>[2x]MITDLADNIERLKANDGLKFSQEYESIDPGQQFTWENSNLEVNKPKNRYANVIAYDHSRVILTSIDGVPGSDYINANYIDGYRKQNAYIATQGPLPETMGDFWRMVWEQRTATVVMMTRLEEKSRVKCDQYWPARGTETCGLIQVTLLDTVELATYTVRTFALHKSGSSEKRELRQFQFMAWPDHGVPEYPTPILAFLRRVKACNPLDAGPMVVHCSAGVGRTGCFIVIDAMLERMKHEKTVDIYGHVTCMRSQRNYMVQTEDQYVFIHEALLEAATCGHTEVPARNLYAHIQKLGQVPPGESVTAMELEFK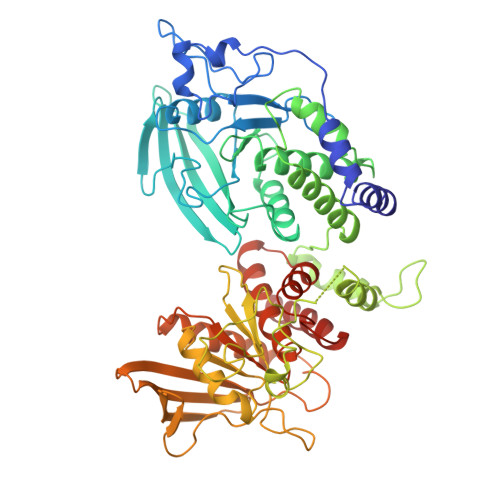LLASSKAHTSRFISANLPCNKFKNRLVNIMPYELTRVCLQPIRGVEGSDYINASFLDGYRQQKAYIATQGPLAESTEDFWRMLWEHNSTIIVMLTKLREMGREKCHQYWPAERSARYQYFVVDPMAEYNMPQYILREFKVTDARDGQSRTIRQFQFTDWPEQGVPKTGEGFIDFIGQVHKTKEQFGQDGPITVHCSAGVGRTGVFITLSIVLERMRYEGVVDMFQTVKTLRTQRPAMVQTEDQYQLCYRAALEYLGSFDHYAT> SQTVDLSCLSGTTVRFFGPSHHFGGFTPLYDPAPDKRVATVDAGANALFIGGGGLNGQFAKTLLEEAEKHGIRLTPEE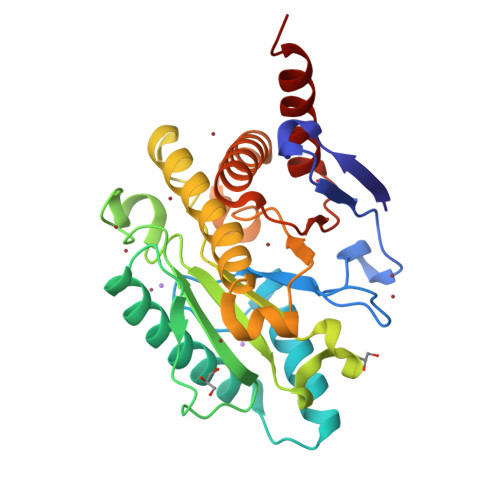LSQHSQRIQQSLLRRAVKSPGKLVELDTGVASPVFARSFGFVPVVPGLMWEESEVGPNVGVTFVHILKPEVTPYGNLNNNVMMYTVAPSGAAPDKTYSLAYKTTIAGVIGAAAAYNDTPAGQQYPVQGLRLPLLGGGIFRRNRSLESIGRANAEGTSLAITRYGPNFELQYMYDPSNAALHGLQEAESTYLASAA>SKIGINGFGRIGRLVLRTALEMGAQVVAVNDPFIALEYMVYMFKYDSTHGMFKGEVKVEDGALVVDGKKITVFNEMKPENIPWSKAGAEYIVESTGVFTTIEKASAHFKGGAKKVIISAPSADAPMFVCGVNLEKYSKDMKVVSNASCTTNCLAPVAKVLHENFEIVEGLMTTVHAVTATQKTVDGPSAKDWRGGRGAAQNIIPSSTGAAKAVGKVIPELDGKLTGMAFRVPTPNVSVVDLTVRLGKECSYDDIKAAMKTASEGPLQGVLGYTEDDVVSCDFT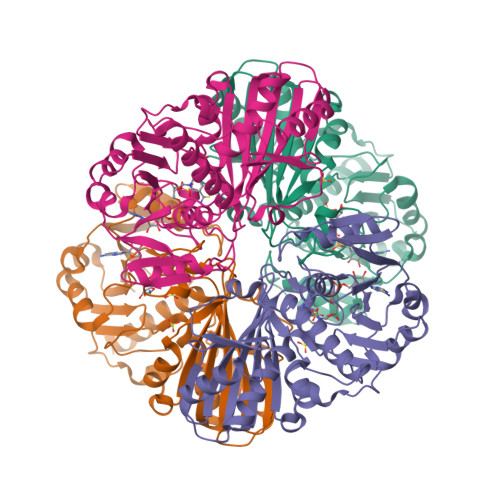GDNRSSIFDAKAGIQLSKTFVKVVSWYDNEFGYSQRVIDLIKHMQKVDSA[4x]O-benzylhydroxylamine | C7 H9 N O | 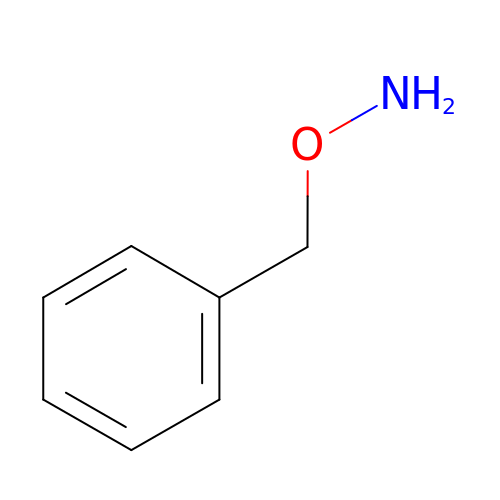XYEOALKITRFCJJ-UHFFFAOYSA-N> METGNKYIEKRAIDLSRERDPNFFDNADIPVPECFWFMFKNNVRQDAGTCYSSWKMDK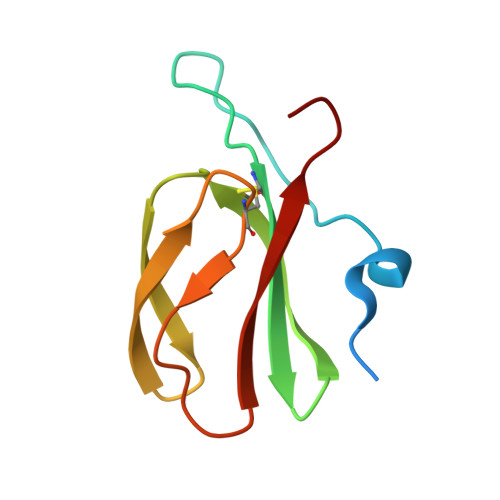KVGPNWVHIKSDDNCNLSGDFPPGWIVLGKKRPGF>MSLSSKLRLQLDAHASI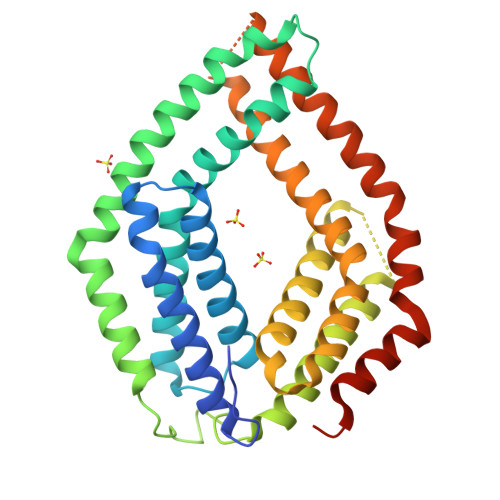HENVRRLLQFTTSIMEANEEGIRKDIDSEFLHDFRVAIRRSRSILRLLNGVFDPEKTAWMLAGLRELGKRTNDLRDSDVYLLRREEYTSLLPPSLRPALDPFFSDLEADKRLHHRQFCRYLTGREYSGFMTSLKEFIAEGELPDPETAPLAAEPTGDVAAKTIRKALKKVLVHGRRTGSETSDAELHELRIDCKKLRYLLEFFASLFPPKATAQVLRQMKTLQDNLGTFVDLTVQMEFLQSRLETIPADRGGISEAAAIGGLLTTLYRKREKVREHFHEIFSGFDSNETGELFDELLTGLAEGHHHHHH[2x]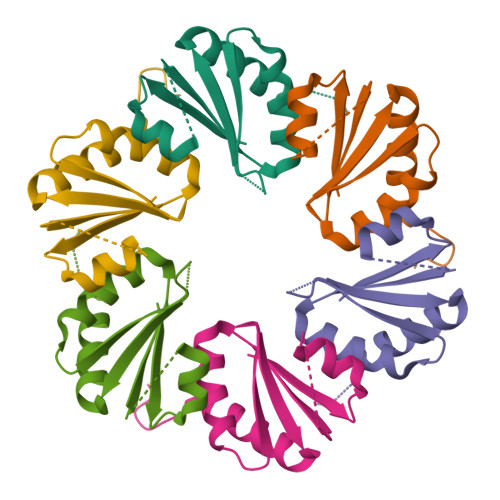>[4x]MEYRIIKSPTQGTIDILCRRKGSGPSKPIGQADAIGLIQGRMIEMVCAADVAEKAVGVTVEDIRGSCPQNMILLAIFGDTASVEAAMDEIRKKETEAGEGWLEHHHHHH> ALPQTVRIGTDTTYAPFSSKDAKGEFIGFDIDLGNEMCKRMQVKCTWVASDFDALIPSLKAKKIDAIISSLSITDKRQQEIAFSDKLYAADSRLIAAKGSPIQPTLESLKGKHVGVLQGSTQEAYANDNWRTKGVDVVA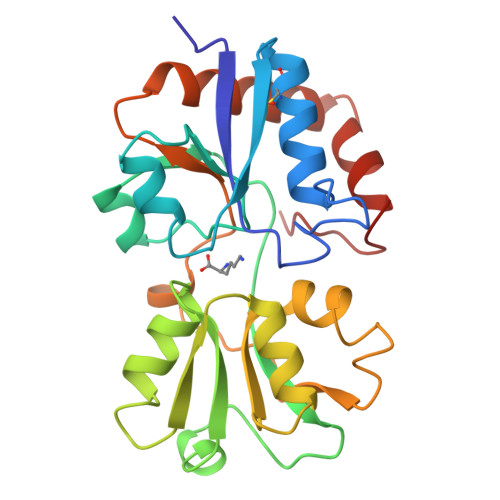YANQDLIYSDLTAGRLDAALQDEVAASEGFLKQPAGKEYAFAGPSVKDKKYFGDGTGVGLRKDDTELKAAFDKALTELRQDGTYDKMAKKYFDFNVYGDK> DKPFNLRSRDPIYSNNYGKLYEITPEKNSQLRDLDILLNCLQMNEGALFVPHYNSRAT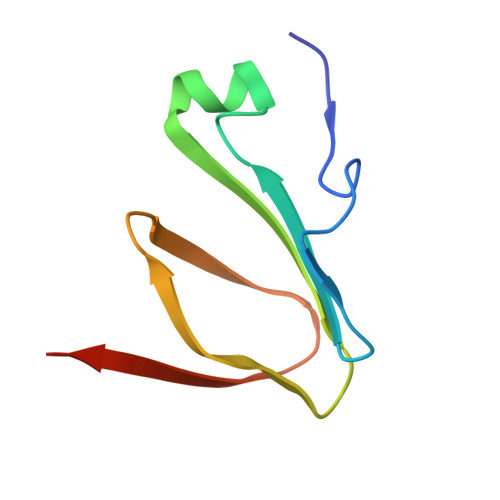VILVANEGRAEVELVGLEQQQ> MQFSKMHGLGNDFVVVDGVTQNVFFTPETIRRLANRHCGIGFDQLLIVEAPYDPELDFHYRIFNADGSEVSQCGNGARCFARFVTLKGLTNKKDISVSTQKGNMVLTVKDMNQIRVNMGEPIWEPAKIPFTANKFEKNYILRTDIQTVLCGAVSMGNPHCVVQVDDIQTANVEQLGPLLESHERFPERVNAGFMQIIN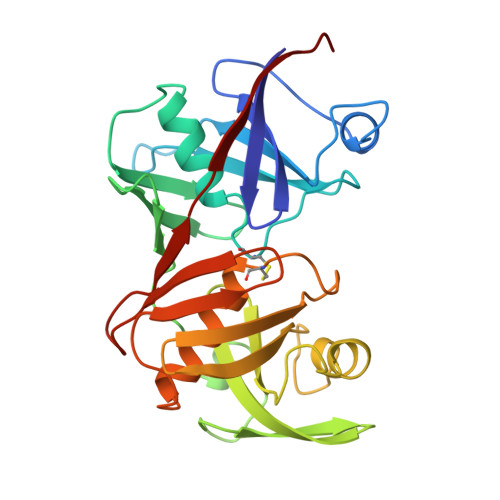KEHIKLRVYERGAGETQACGSGACAAVAVGIMQGLLNNNVQVDLPGGSLMIEWNGVGHPLYMTGEATHIYDGFITL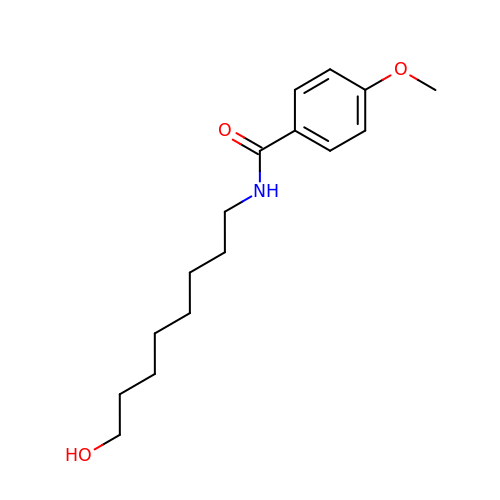N-(8-hydroxyoctyl)-4-methoxybenzamide | C16 H25 N O3 | NQLXMEWCEUVFAX-UHFFFAOYSA-N[(2R,3S,4R,5R)-3,4,5-tris(oxidanyl)oxan-2-yl]methyl dihydrogen phosphate | C6 H13 O8 P | 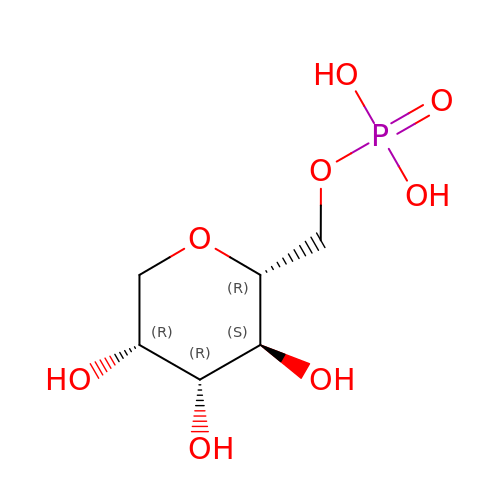KAJAXXUCVJFKFM-KVTDHHQDSA-N> KRNKPGKATGKGKPVNNKWLNNAGKDLGSPVPDRIANKLRDKEFKSFDDFRKKFWEEVSKDPELSKQFSRNNNDRMKV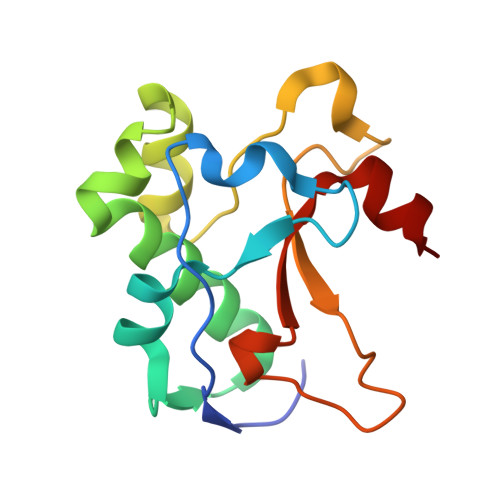GKAPQTRTQDVSGKRRSFELHHEKPISQNGGVYDMDNISVVTPKRAIDIH> RQWALEDFEIGRPLGKGKFGNVYLAREKQSKFILALKVLFKAQLEKAGVEHQLRREVEIQSHLRHPNILRLYGYFHDATRVYLILEYAPLGTVYXELQKLSKFDEQRTATYITELANALSYCHSKRVIHRDIKPENLLLGSAGELKIADFGWSVHAPSSRRTTLAGTLDYLPPEMIEGRMHDEKVDLWSLGVLCYEFLVGKPP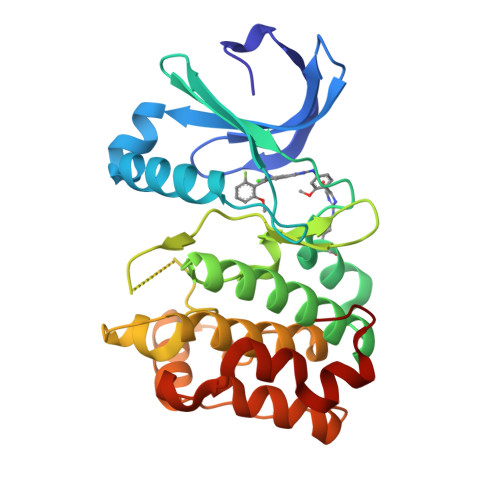FEANTYQETYKRISRVEFTFPDFVTEGARDLISRLLKHNPSQRPMLREVLEHPWITANSSKPS> MGSSH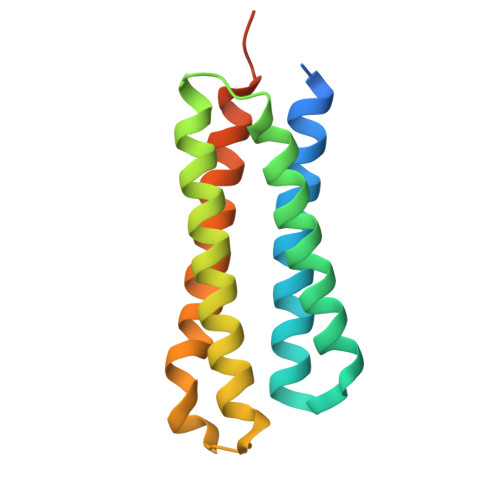HHHHHQGSMLNNMLITNEIKQHVDSSLDNFNQYILNGTPSKKESYNNEVILAKQKIGNLKKNSDDVNQYILRDLDNTLDSYIESSKNTISAYENKEGYVFYYDDFVAAKNIASYCDAYASTLMQNFLEANSIAYKELNRNSS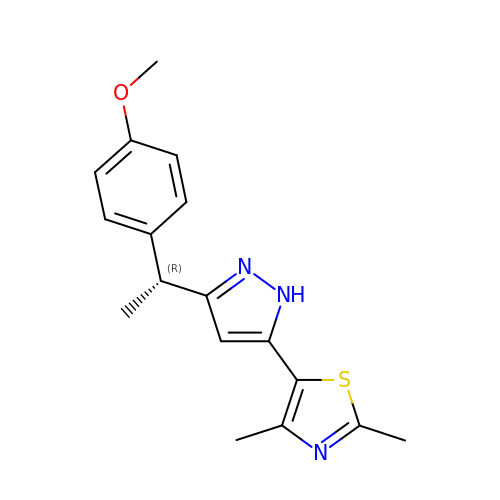5-{3-[(1R)-1-(4-methoxyphenyl)ethyl]-1H-pyrazol-5-yl}-2,4-dimethyl-1,3-thiazole | C17 H19 N3 O S | ABGBHHDSOIOYML-SNVBAGLBSA-N(2S)-2-[3-(AMINOMETHYL)PHENYL]-3-{(S)-HYDROXY[(1R)-2-METHYL-1-{[(2-PHENYLETHYL)SULFONYL]AMINO}PROPYL]PHOSPHORYL}PROPANOIC 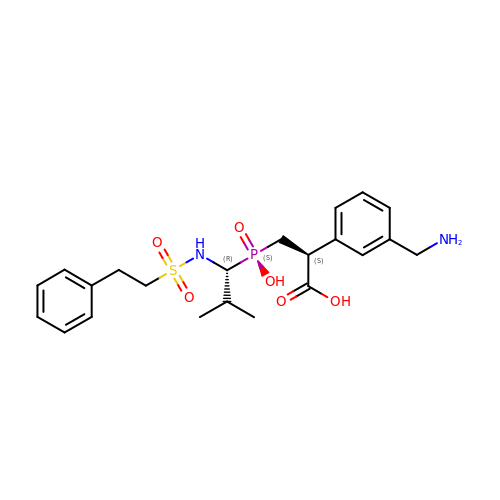ACID | C22 H31 N2 O6 P S | CTQDLSDUHUFBQW-LEWJYISDSA-N> MSHYHEQFLKQNPLAVLGVLRDLHKAAIPLRLSWNGGQLISKLLAITPDKLVLDFGSQAEDNIAVLKAQHITITAETQGAKVEFTVEQLQQSEYLQLPAFITVPPPTLWFVQRRRYFRISAPLHPPYFCQTKLADNSTLRFRLYDLSLGGMGALLETAKPAELQEGMRFAQIEVNMGQWGVFHFDAQLISISERKVID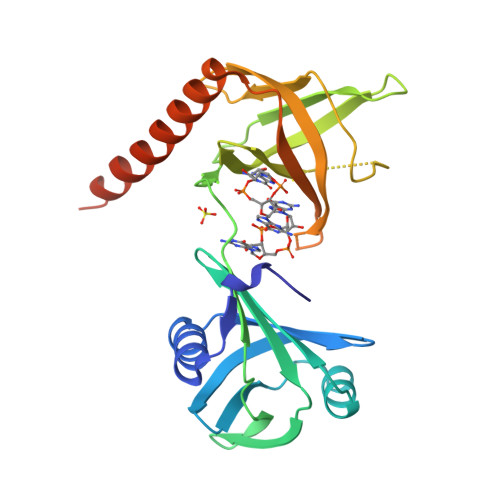GKNETITTPRLSFRFLNVSPTVERQLQRIIFSLEREAREKADKVRDKLAAALEHHHHHH>[2x]XEVEALEA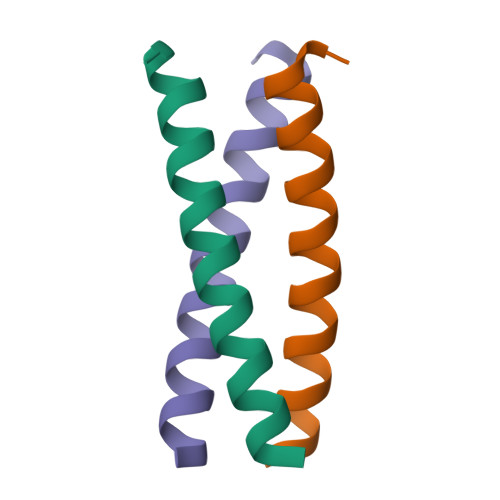KVEALEYKVQKLEKKVEALEHGW>[2x]KCLALLAAVASL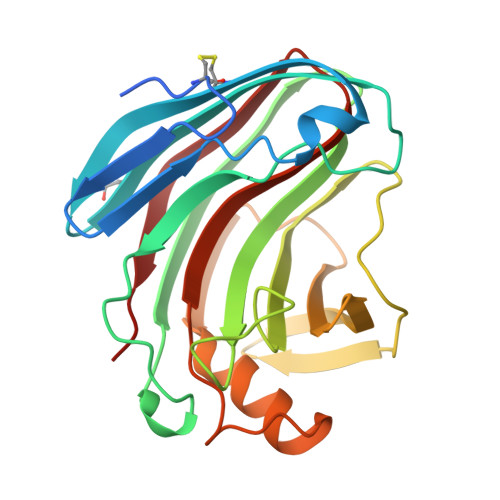GSAQQLCEQYGYHAANGYYFNNNMWGQGSGSGSQCLTVDSAQSGGVSWHVDWQWSGGQNNVKSYPYAGRELPQKRLVSSIGSIPTSASWGYSGNNLRANVAYDLFTAADPNHETSSGDYELMIWLGRLGDVYPIGSSVGFVNVGGQQWELFDGYNGNMHVFSFVAPQQINNFNTDVKTFFDYLTWNRGFPADQQHLLILQFGTEPFTGGPATFQVNHFSGQVN(2'S,3R,4'S,5'R)-N-(4-carbamoylphenyl)-6-chloro-4'-(3-chloro-2-fluorophenyl)-2'-(2,2-dimethylpropyl)-2-oxo-1,2-dihydrospiro[indole-3,3'-pyrrolidine]-5'-carboxamide 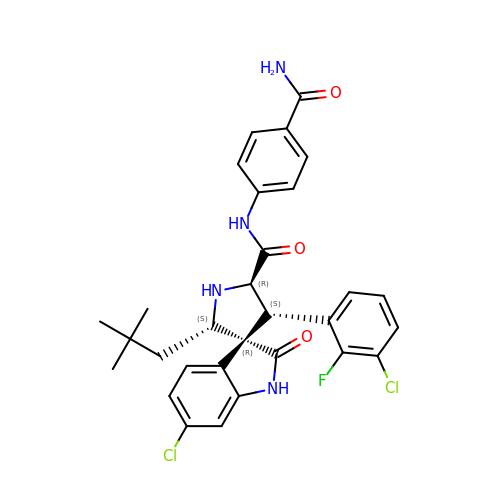| C30 H29 Cl2 F N4 O3 | KALNCVZAFDQICX-AMKZZFPWSA-N> MAGNLVSWACKLCRSPEGFGPISFYGDFTQCFIDGVILNLSAIFMITFGIRDLVNLCKKKHSGIKYRRNWIIVSRMALVLLEIAFVSLASLNISKEEAENFTIVSQYASTMLSLFVALALHWIEYDRSVVANTVLLFYWLFETFGNFAKLINILIRHTYEGIWYSGQTGFILTLFQVITCASILLLEALPKKPLMPHQHIHQTLTRRKPNPYDSANIFSRITFSWMSGLMKTGYEKYLVEADLYKLPRNFSSEELSQKLEKNWENELKQKSNPSLSWAICRTFGSKMLLAAFFKAIHDVLAFTQPQLLRILIKFVTDYNSERQDDHSSLQGFENNHPQKLPIVRGFLIAFAMFLVGFTQTSVLHQYFLNVFNTGMYIKSALTALIYQKSLVLSNEASGLSSTGDIVNLMSVDVQKLQDLTQWLNLIWSGPFQIIICLYSLYKLLGNSMWVGVIILVIMMPLNSFLMRIQKKLQKSQMKYKDERTRVISEILNNIKSLKLYAWEKPYREKLEEVRNNKELKNLTKLGCYMAVTSFQFNIVPFLVSCCTFAVFVYTEDRALTTDLVFPALTLFNLLSFPLM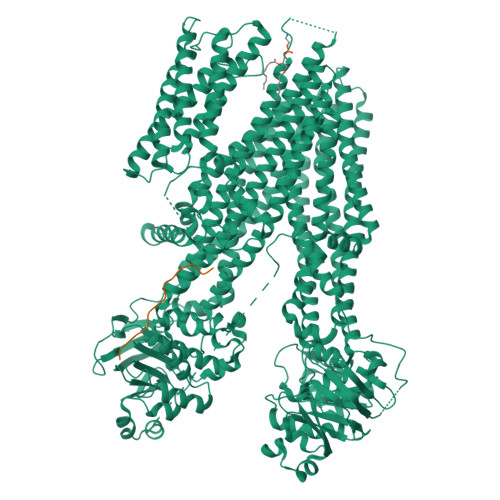IIPMVLNSFIEASVSIGRLFTFFTNEELQPDSVQRLPKVKNIGDVAINIGDDATFLWQRKPEYKVALKNINFQAKKGNLTCIVGKVGSGKTALLSCMLGDLFRVKGFATVHGSVAYVSQVPWIMNGTVKENILFGHRYDAEFYEKTIKACALTIDLAILMDGDKTLVGEKGISLSGGQKARLSLARAVYARADTYLLDDPLAAVDEHVARHLIEHVLGPNGLLHTKTKVLATNKVSALSIADSIALLDNGEITQQGTYDEITKDADSPLWKLLNNYGKKNNGKSNEFGDSSESSVRESSIPVEGELEQLQKLNDLDFGNSDAISLRRASDATLGSIDFGDDENIAKREHREQGKVKWNIYLEYAKACNPKSVCVFILFIVISMFLSVMGNVWLKHWSEVNSRYGSNPNAARYLAIYFALGIGSALATLIQTIVLWVFCTIHASKYLHNLMTNSVLRAPMTFFETTPIGRILNRFSNDIYKVDALLGRTFSQFFVNAVKVTFTITVICATTWQFIFIIIPLSVFYIYYQQYYLRTSRELRRLDSITRSPIYSHFQETLGGLATVRGYSQQKRFSHINQCRIDNNMSAFYPSINANRWLAYRLELIGSIIILGAATLSVFRLKQGTLTAGMVGLSLSYALQITQTLNWIVRMTVEVETNIVSVERIKEYADLKSEAPLIVEGHRPPKEWPSQGDIKFNNYSTRYRPELDLVLKHINIHIKPNEKVGIVGRTGAGKSSLTLALFRMIEASEGNIVIDNIAINEIGLYDLRHKLSIIPQDSQVFEGTVRENIDPINQYTDEAIWRALELSHLKEHVLSMSNDGLDAQLTEGGGNLSVGQRQLLCLARAMLVPSKILVLDEATAAVDVETDKVVQETIRTAFKDRTILTIAHRLNTIMDSDRIIVLDNGKVAEFDSPGQLLSDNKSLFYSLCMEAGLVNENDYKDHDGDYKDHDIDYKDDDDK> SWVWNQMFVLEEFSGPEPILVGRLHTDLDPGSKKIKYILSGDGAGTIFQINDITGDIHAIKRLDREEKAEYTLTAQAVDFETNKPLEPPSEFIIKVQDINDNAPEFLNGPYHATVPEMSILGTSVTNVTATDADDPVYGNSAKLVYSILEGQPYFSIEPETAIIKTALPNMDREAKEEYLVVIQAKDMGGHSGGLSGTTTLTVTLTDVNDNPPKFAQSLYHFSVPEDVVLGTAIGRVKANDQDIGENAQSSYDIIDGDGTA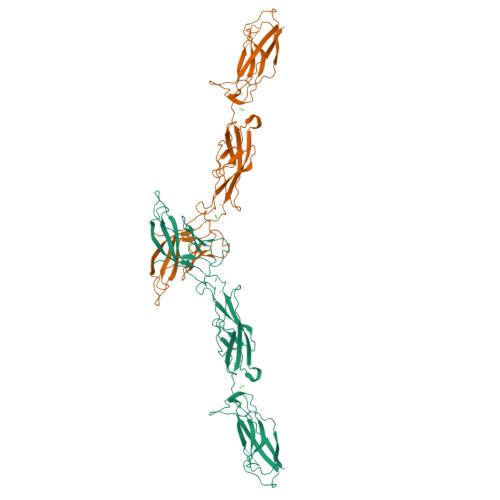LFEITSDAQAQDGVIRLRKPLDFETKKSYTLKVEAANIHIDPRFSSRGPFKDTATVKIVVE> ADLPMMPPVGVQASILSHDTIRITWADNSLPKHQKITDSRYYTVRWKTNIPANTKYKNANATTLSYLVTGLKPNTLYEFSVMVTKGRRSSTWSMT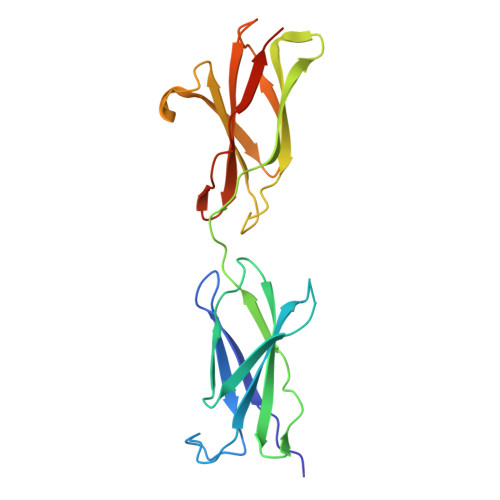AHGTTFELVPTSPPKDVTVVSKEGKPKTIIVNWQPPSEANGKITGYIIYYSTDVNAEIHDWVIEPVVGNRLTHQIQELTLDTPYYFKIQARNSKGMGPMSEAVQFRTPKAHHHHHH> MAFELFTPLFNKIDQTTATYVTDISSRAIAAITPVVSVGL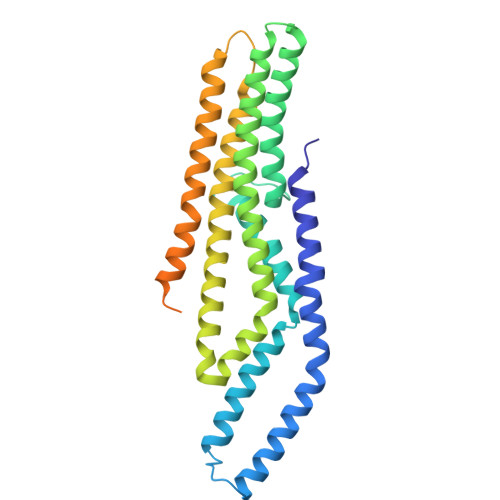TLGFITYGWLIIRGAVEMPVAEFLNRCLRIGIIVSIALAGGLYQGEIANAITTVPDELASALLGNPTQGASAAALVDQSAQQGFDRASEAFEEAGFFSSDGLLYGLFGIIILLATGLLAAIGGAFLLLAKIALALLAGLGPLFILALIWQPTHRFFDQWAQQVLNYGLLIVLFAAVFGLLMQIFGSYMADLRFDGAQNVAYAIGGSVILSIVSIVLLMQLPSIASGLAGGIGLGYMWELRSMRSGAGAAMRGGRAMARGARAAPGAARGAAVGAANMAKTVATGGAGVARAAAGYFRGRKAG> MRKNLFAKRAVAFLLGIVITAAGIVSFNTVSTSAAGEYNYAKALQYSMFFYDANMCGTGVDENSLLSWRGDCHVYDARLPLDSQNTNMSDGFISSNRSVLDPDGDGKVDVSGGFHDAGDHVKFGLPEAYAASTVGWGYYEFKDQFRATGQAVHAEVILRYFNDYFMRCTFRDASGNVVAFCHQVGDGDIDHAFWGAPENDTMFRRGWFITKEKPGTDIISATAASLAINYMNFKDTDPQYAAKSLDYAKALFDFAEKNPKGVVQGEDGPKGYYGSSKWQDDYCWAAAWLYLATQNEHYLDEAFKYYDYYAPPGWIHCWNDVWSGTACILAEINDLYDKDSQNFEDRYKRASNKNQWEQIDFWKPIQDLLDKWSGGGITVTPGGYVFLNQWGSARYNTAAQLIALVYDKHHGDTPSKYANWARSQMDYLLGKNPLNRCYVVGYSSNSVKYPHHRAASGLKDANDSSPHKYVLYGALVGGPD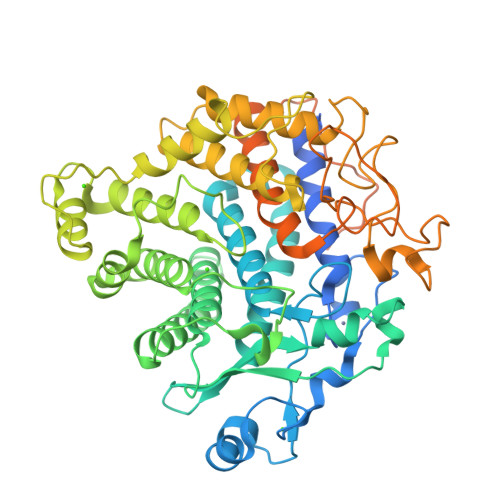ASDQHVDRTNDYIYNEVAIDYNAAFVGACAGLYRFFGDSSMQIDPSMPSHNVPVPPTPTPPDTQIVYGDLNGDQKVTSTDYTMLKRYLMKSIDRFNTSEQAADLNRDGKINSTDLTILKRYLLYSIPSLPI> XK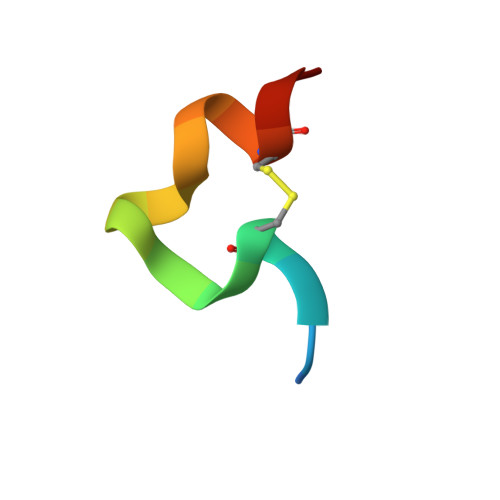GHPCDYPEWQWLCELX> TGGSVHSSPAIG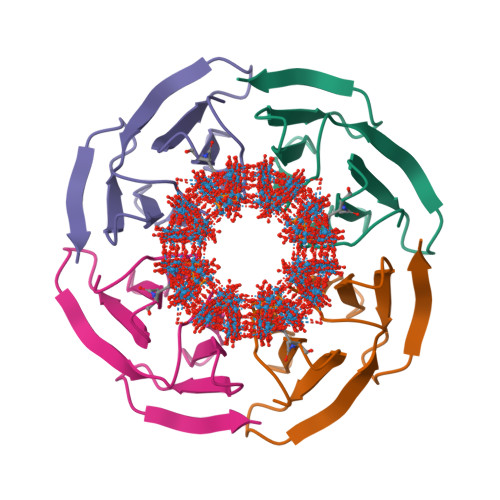QDGTIYVGSNDHYLYAINPNGKLKWKFETGGSVHSSPAIGQDGTIYVGSNDHYLYAINPNGKLKWKFE> NMMEY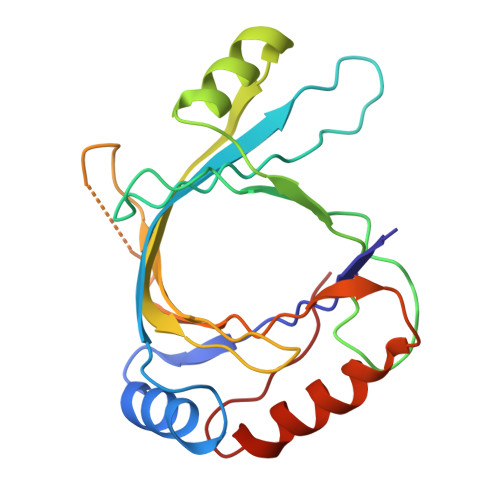LLQGSVLDHSLESLIHRLRGLCDNMEPETFLDHEMVFLLKGQQASPFVLRARRSMDRAGAPWHLRYLGQPEMGDKNRHALVRNCVDIATSENLTDFLMEMGFRMDHEFVAKGHLFRKGIMKVVVYKIFRILVPGNTDSTEALSLSYLVELSVVAPAGQDMVSDDMRNFAEQLKPLVHLEKID>[3x]GSHMASNKYKRIFLVVMDSVGIGEAPDAEQFGDLGSDTIGHIAEHMNGLQMPNMVKLGLGNIREMKGISKVEKPLGYYTKMQEKSTGKDQMTGHWEIMGLYIDTPFQVFPEGFPKELLDELEEKTGRKIIGNKPASGTEILDELGQEQMETGSLIVYTSADSVLQIAAHEEVVPLDELYKICKIARELT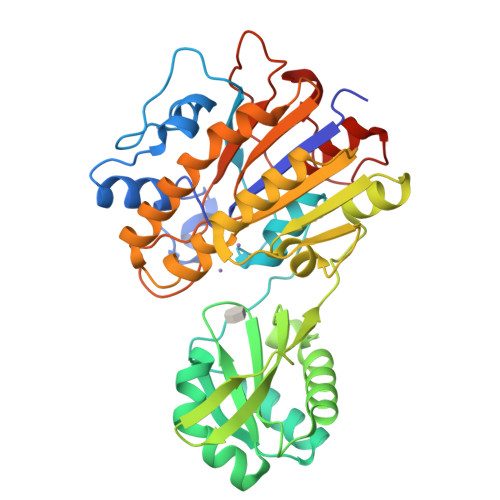LDEKYMVGRVIARPFVGEPGNFTRTPNRHDYALKPFGRTVMNELKDSDYDVIAIGKISDIYDGEGVTESLRTKSNMDGMDKLVDTLNMDFTGLSFLNLVDFDALFGHRRDPQGYGEALQEYDARLPEVFAKLKEDDLLLITADHGNDPIHPGTDHTREYVPLLAYSPSMKEGGQELPLRQTFADIGATVAENFGVKMPEYGTSFLNELKK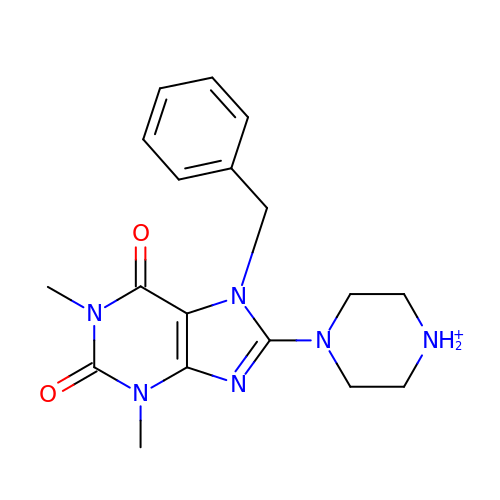7-BENZYL-1,3-DIMETHYL-8-PIPERAZIN-1-YL-3,7-DIHYDRO-PURINE-2,6-DIONE | C18 H23 N6 O2 | QFSMMXJBEBXTJP-UHFFFAOYSA-O> HMEQGICGSHVFFIEDGKSKNYIIGKYKIGYLSGDNLILDPYECLYLYF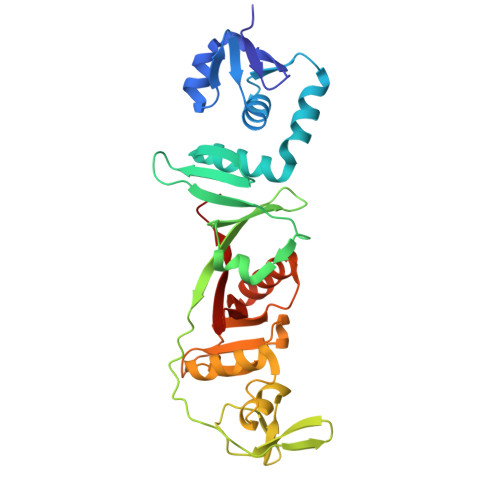KGRISFQNSDSFRDLFDTVTFDRYVAYEILKNKGYRVKEDSGLIYFRKGTEKPLSLRVMREYDRIQFSDLVENPVDYYFTVDEEGDPTVYSSQEIFPGGRNLVSPVSAPVVRMGGRSFGAGDLEWWIGTAFHGFRLLTENEANYISGNHSASQVDMVYSDLVGRGCIVKTGFKYGANFRVYLGRDSQHAEYLVSVMPEEERWYSISRGVRVASSVRKTMIYASIYKNEVRYVALKRVKDII>MGKAVIAIHGGAGAISRAQMSLQQELRYIEALSAIVETGQK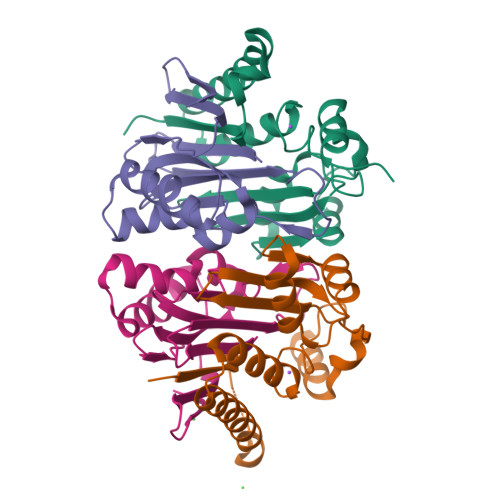MLEAGESALDVVTEAVRLLEECPLFNAGIGAVFTRDETHELDACVMDGNTLKAGAVAGVSHLRNPVLAARLVMEQSPHVMMIGEGAENFAFARGMERVSPEIFSTSLRYEQLLAARKEGATVLDHSGAPLDEKQKMG[2x];>TVGAVALDLDGNLAAATSTGGMTNKLPCTVGAAPLVGAGCYANNASVAVSCTGTGEVFIRALAAYDIAALMDYGGLSLAEACERVVMEKLPALGGSGGLIAIDHEGNVALPFNTEGMYRAWGYAGDTPTTGIYREKGDTVATQ[2x]> MGGAHKVRAGGPGLERAEAGVPAEFSIWTREAGAGGLAIAVEGPSKAEISFEDRKDGSCGVAYVVQEPGDYEVSVKFNEEHIPDSPF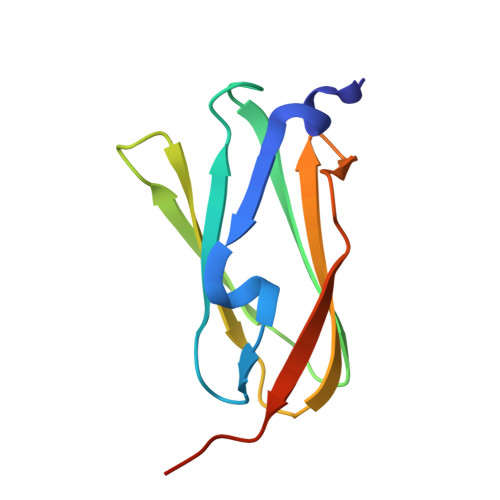VVPVASPSGGGGGG>MTQSEDIKWGMFLNTARPPQFTERRVLEN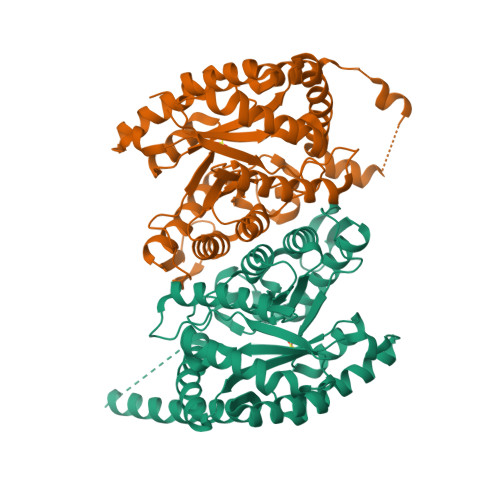AKFYGQVAEEMGFESAWMLEHHFTDYGLCGSPMVMASYILGATRRIKVGTAINILPLEHPVRLAEQAALLDQLSDGRFILGIGRGFFDKDFTVFGVDIHDTRALTHNYYDIMQEAWTKGVVGSDGPFLNFPPVPVNPRPYSDKMPMVCAAMSPSTIEWAAKNGLPMIMQHDIEHNEKASNVELYRALAEEHGHDPDGIEHTIAMIVAVDPDRERVREECRHYLNWFEDAVEKAQNIIDIVREHGVECYDWHLRKWREAVIKGDTAISKVVDNLLRLNAIGTPEDAIETIQHVIDVTGVKRVVVGFEAIGDRDRVLESMKLFDEQVRPHIRGAKIGSHHHHHH[4x]> TG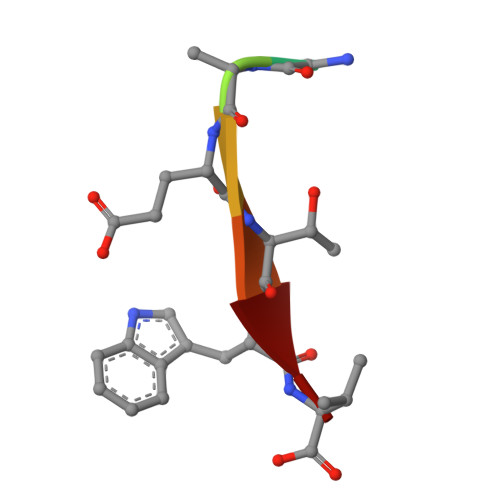YETWV>MHHHHHHMELSLASITVPLESIKPSNILPVTVYDQHGFRILFHFARDPLPGRSDVLVVVVSMLSTAPQPIRNIVFQSAVPKVMKVKLQPPSGTELPAFNPIVHPSAITQVLLLANPQKEKVRLRYKLTFTMGDQTYNEMGDVDQFPPPETWGSL[2x];>DDDDFGGFEAAE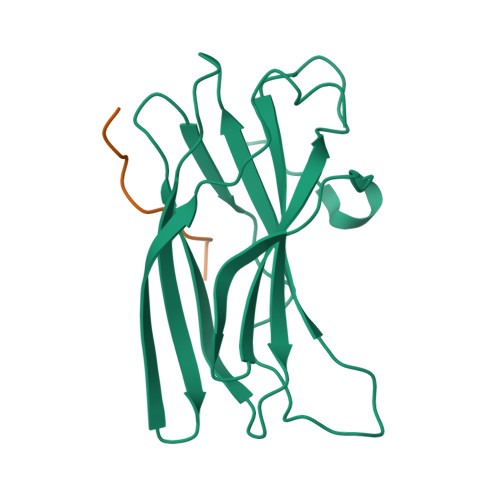TFD[2x]>[8x]GUUUAUAGACAUAGCCUUGUGUAUGACUGUCUAAUCAACAGUGCAAGGAAUUAGUUGUGCUCUCAAAAGGAGUUAUGUGAAGGAAAGAUUAAAUGGAUACAUUUAAUUAAGUACAAUUACUACAAAAUCUAUAAUGACUGGGUAAGUCACCCGUAAGAAGGAUGAGUUAGUAGAGAUAUAAUAAUAUCUUACAGUUCAAC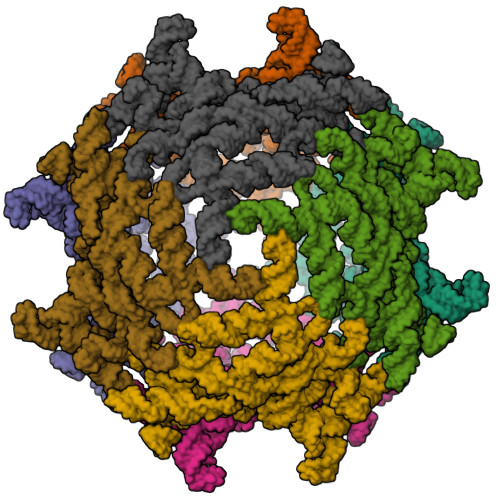UGAUGUGCAAGUUUAUAAGUAGACGUAGUGUGAAAGACUUAUCGCUAACGCAAUAGACGUUAUCUCGAAAGGAUAAAAGAAACCAAGAAGAUAUACAAAUUGGUAACUUGUAUAAGCCCUUGGUAAUACCAAAUAAGUUAGUUCCUCAUGAUGUCGUGGAAACAUGACUAUAAGAUAAGUUGAAUUCGAUAGUAGCCCAAGAGGAAUCNNNNNNNNNNNNNNNNNNNNNNNNNNNNNNNNNNNNNNNNNNNNNNNNNNNXGAUUGUGCCUUGAAAAAGGUGGGUGAGGUCUGUGGGUAAAAAUUAAUUCCCAUCUGGUUUUGGAUUUUCUUCGGAAAAUUGGUGCAAGAAGCGUGGAGUUGCUAACCAUUGCUCAGACUUGUAUCGCCAGUAGCACGAUAACGAUAUUUAUGAAUGUUGUAAGGUGAAUAAAAGCCUAUGAUUUGUGAAC> MGHHHHHHLYFQGMNRPSFNEAWLAFRKVNHSVADVGSIIGGNVGKNITGGYFQNACPIRMSYVLNATGFPIARNSPYAKVSGADNKFYIYRVNDMIDYLTHTMGKPDLIVNNPKQSDFIGKKGIIVV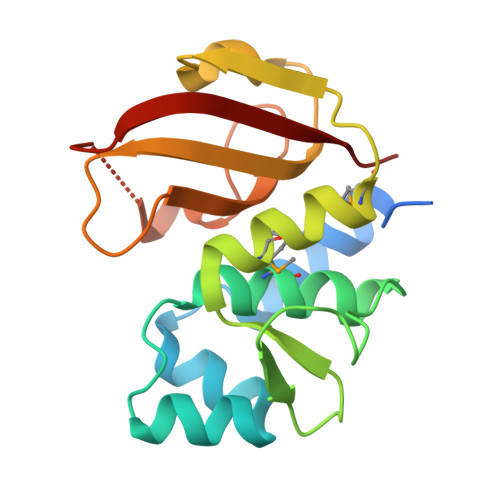KGHGWSNARGHVTLWNGSICSDQCHLLNDPDNGPFVPEVGTLWILP> MTPHLMKLLGLSAALLAISQG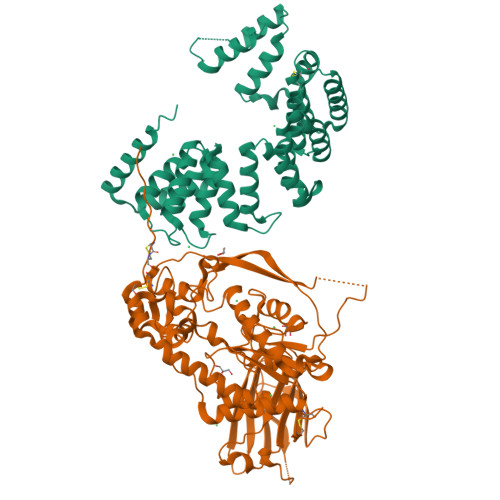VRAEDVKAPTFSAEPCCQLCPEAHDASRYTTRYQQNFTTLVQAQGDWLFRTREDLRTEFNTTPAGYKRLQQVHDAFKKRGVELVVVYQPTRGLVNRNMLNPAEKAAFDYQKALGNYQAMLKRFASMGYNVPDLSPLTNEQLAAADQGKDFYFRGDQHWTPYGAERAAKIVADTVHKMPAFEGIPRKEFETRKSGRMGKTGTLHNVAGQLCGTSYAVQYMDQFATEPKGASGGDDLFGDSGNAQITLVGTSHSGKNYNFSGFLEQYIGADVLNVAFPGGGLEGSMIQYLGSEEFQKNPPKILIWEFSPLYRLDQETIWRQILGLLDDGCDDRPALMSASTTLKPGKNELMVNGKGGVIKDLINRNLQMDVKFEDPSVKVLQATLWYLNGRHEDIKLEKPETSDTDGRFVFQMREDEDWASQRLLAFEVQGPESGTQKVEAKLCKRNNFAVPAQTAQAGQLEHHHHHH;> MCAGLPDQRLANEALKRGDTALAERNYKALADLGYSEAQVGLADIKVATRDPSQIKEAEATYRAAAATSPRAQARLGRLLVAKPDSTQAEREEAETLLKQAAKQGQSNTLIPLAMLYLSYPQSFPKVNAQQQIDQWRAAGNPEAGLAQVLLYRTQGTYDQHLGEVEKICKAALNTTDICYVELATVYQKRGQADQQAALLGQLKSAYARGAVPATRVDSVARVLADRSLGQTDEKTAKELLEQVAPANPASWVSLAQLVYDFPELGDTDQLMAYIDKGREAEQPRAELLLGRLYYEGKTLPADAQKAEQHLQAAAEAGEISAHYYLGQLYRRGYLGNVEPQKAVDHLLAAARGGQNSADYALAQLFSEGHGIRPQPGNAWVFAQLSQANPTPQSAELLQQLDQQLTPDQRNQAQQLLDQEKRARGSLAQGANSTLALEALQDDEKEVDGEDSLLEHHHHHH2-(dodecyloxy)-6-hydroxybenzoic acid | C19 H30 O4 | 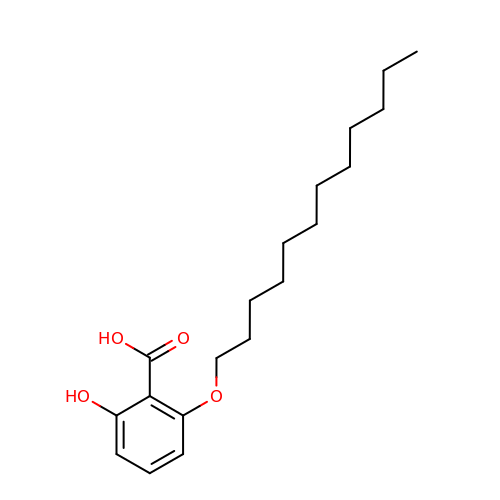HMYWVVRALHTQJQ-UHFFFAOYSA-N>[7x]MAIAQLATEYVFSDFLLKEPTEPKFKGLRLELAVDKMVTCIAVGLPLLLISLAFAQEISIGTQISCFSPSSFSWRQAAFVDSYCWAAVQQKNSLQSESGNLPLWLHKFFPYILLLFAILLYLPPLFWRFAAAPHICSDLKFIMEELDKVYNRAIKAAKSARDLDMRDGACSVPGVTENLGQSLWEVSESHFKYPIVEQYLKTKKNSNNLIIKYISCRLLTLIIILLACIYLGYYFSLSSLSDEFVCSIKSGILRNDSTVPDQFQCKLIAVGIFQLLSVINLVVYVLLAPVVVYTLFVPFRQKTDVLKVYEILPTFDVLHFKSEGYNDLSLYNLFLEENISEVKSYKCLKVLENIKSSGQGIDPMLLLTNLGMIKMDVVDGKTPMSAEMREEQGNQTAELQGMNIDSETKANNGEKNARQRLLDSSCLEWSHPQFEK

Pannexin 1 (PANX1) plays extensive physiological roles across diverse fields of biology, including cell death, inflammation, cancer progression, and neurological disorders. As suggested by biochemical analysis, PANX1 forms an oligomeric channel for the facilitated diffusion of ions and large molecules across the plasma membrane upon activation. The overall structure of human PANX1 presents a novel heptameric assembly, which is distinct from gap junction channels (connexins and innexins)8,9 and functionally related channels, such as CALHM and LRRC8. Interestingly, the protomer of PANX1 shares a similar fold of four transmembrane helices with the aforementioned channels.

Caspase 3-mediated cleavage of the cytoplasmic CT tail irreversibly activates PANX1 and triggers the release of the “find-me” signaling molecule for dying cell clearance. Cleavage at the S2 site is essential for the activation of PANX1.1 We generated CT-cleaved PANX1, named PANX1ΔCT, via Drosophila effector caspase (drICE) cleavage. As shown by SDS-PAGE, PANX1ΔCT was partially cleaved by drICE at the S1 site, and this result is consistent with caspase 3 cleavage. However, the dramatically deferred monodisperse peak of PANX1ΔCT observed by gel filtration (~1–1.5 mL) indicated that PANX1ΔCT underwent a large conformational change or that reasonable disorder regions were removed. 3 pA, whereas incorporation of PANX1ΔCT resulted in the channel opening up to 177 pA under +100 mV. We therefore collected the cryo-EM dataset for PANX1ΔCT and solved its structure at 3.1 Å resolution following a similar image processing strategy as the full-length dataset. Surprisingly, the two structures revealed almost identical conformations except that the density of the intracellular region of PANX1ΔCT was weaker. Interestingly, the channel gating was observed in PANX1ΔCT, which indicated PANX1ΔCT was highly dynamic under the condition of electrophysiological study. However, it is still not sufficient to stabilize PANX1ΔCT in a distinct conformation under the condition of cryo-EM sample preparation.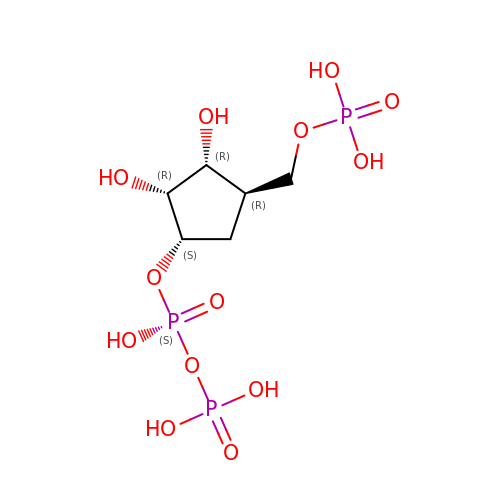1-ALPHA-PYROPHOSPHORYL-2-ALPHA,3-ALPHA-DIHYDROXY-4-BETA-CYCLOPENTANE-METHANOL-5-PHOSPHATE | C6 H15 O13 P3 | OICBXEWBKALHHB-MOJAZDJTSA-N> DACTLLAP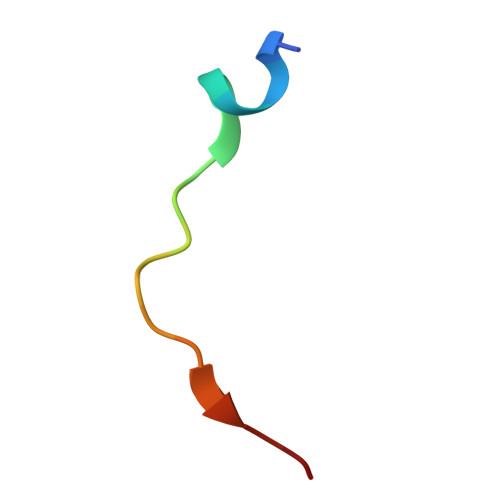AAGDTIISLCF> MEKVYQAGTHEGMIDFINMEDLELAATQVIPSGGYGYISSGAGDLFTYRENQKAFNHQLVIPHVLKDVELPDTTTYFSDETLAAPIIMAPVAAHGLAHEQAEKASAKGVSEFGTIYTASSYASCTLEEIRAAGGPEA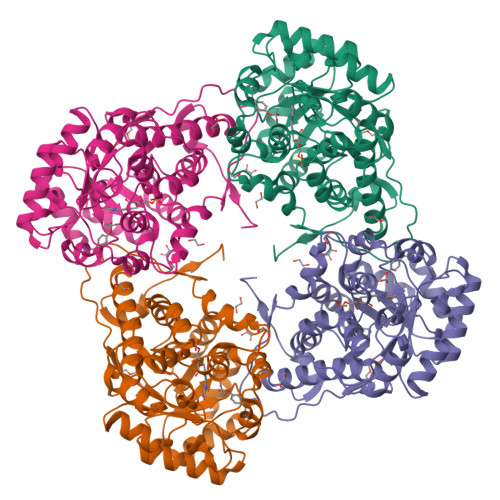PQWFQFYMSKDDGINLDILEMAKRNGAKAVVLTADATVGGNRETDRRNGFTFPLPMPIVQAYQSGVGQTLDAVYKSSKQKLSPKDIEFITTHSELPVYVKGVQSEDDVYRSLDAGAQGIWVSNHGGRQLDGGPASFDSLRYVAEAVDKRVPIVFDSGVRRGQHIFKAIASGADLVAIGRPAIYGLSLGGSTGIKQVFDFFKTELEMVMQLAGTQTVEDIKNAKLRENRFMC> MPQIVFTATALRDLERLREFLRSKNPPAAQRAASAIINTIRKLESYPDIGRPIDDNDF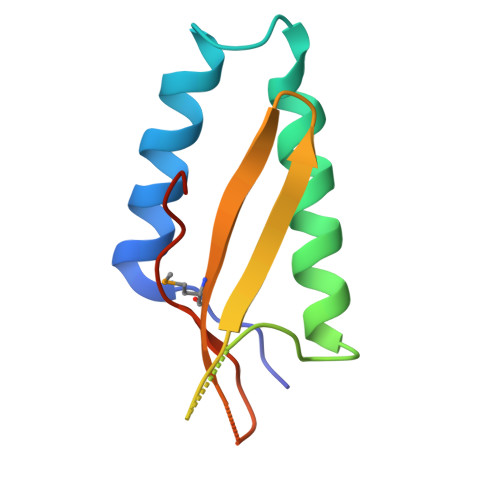SFRELLIDFGDTGYLAMYQYDGGERLTVLCIRHQKEAGY Flcn is also known to have two paralogous binding partners, the Flcn interacting partners Fnip1 and Fnip2, which interact independently with Flcn. This Flcn/Fnip (either Flcn/Fnip1 or Flcn/Fnip2) complex has been recently reported to be involved in amino acid sensing through regulation of the Rag GTPases at the lysosomal membrane and therefore controlling signalling through mTORC1. With the motivation to understand more about the Flcn/Fnip complex, we sought to investigate their putative yeast orthologues Lst7 and Lst4. We solved the structure of the Lst4 longin domain, thereby confirming it as a bona fide member of the DENN family. Additionally, we show that Lst4 interacts with Lst7, not through its longin domain but through its DENN domain, and we demonstrate that the Lst7/Lst4 complex exists as a 1 : 1 heterodimer.

In order to overcome this, the Lst4 longin domain from Kluyveromyces lactis, a closely related budding yeast, was expressed, purified and crystallized. The K. lactis longin domain (aa 58–226) crystallized in the P42212 space group with four molecules in the asymmetric unit (AU). The final structure was determined at 2.14 Å resolution by molecular replacement of a higher resolution native dataset. Several loops were missing in the electron density, between β1–β2, β2–α1 and α1–β3, in addition to nine residues at the N-terminus and 13 residues at the C-terminus, most likely owing to their inherent flexibility. The structure reveals the classical architecture of a longin domain, which is the first domain of the complete DENN module. The domain is made up of a core five-strand β-sheet, with one short α-helix (α1) traversing the face of the concave side and the longer α2 and α3 packed against the convex side. An entirely novel feature, which is not present in any other previously determined longin domain structure, is the kinked helical extension to α2. ConSurf analysis of the structure identified two conserved surface regions of the Lst4 longin domain, which were mapped onto a surface representation of the Lst4 longin structure. The first patch (P1) mainly comprises residues from α1 and several that lie on the loop that precedes β3. The four molecules seen in the crystal structure do not represent a biologically relevant assembly, as an analytical ultracentrifugation experiment indicated that the protein was monomeric in solution.

>MGNDRLHNGGFRLIISQELGHVTSRNNYQVVLDHSSVNFHTGAHIPLNELKDYIFGSSIRTIDYSASSDKIKVVKSANIVLFTRIFYLNEKSTLRIAISCCVTDDVLPVLTECWPHISSFLDQCENTLLKYLAKNDTQFLPHDWKARNCIEVAAVLQTFQRKIIPLLSGYSLEGSHHHHHH[4x]>[180x]ASNFTQFVLVDNGGTGDVTVAPSNFANGVAEWISSNSRSQAYKVTCSVRQSSAQNRKYTIKVEVPKVATQTVGGVELPVAAWRSYLNMELTIPIFATNSDCELIV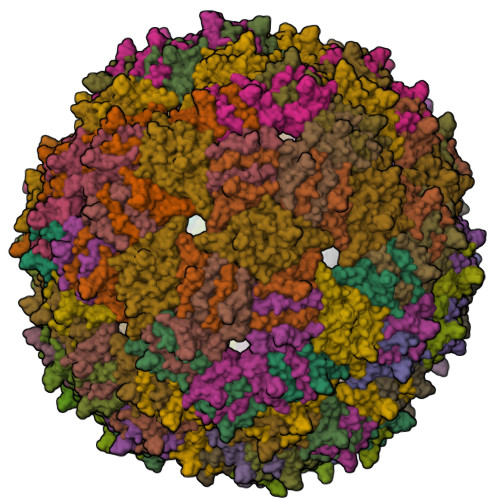KAMQGLLKDGNPIPSAIAANSGIY> GTGCGTGTGACTGT;> CGGACAGTCACACGCA;> ACACCGT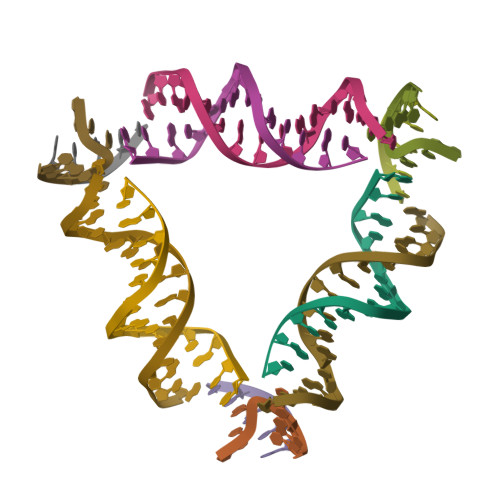;> CTGTA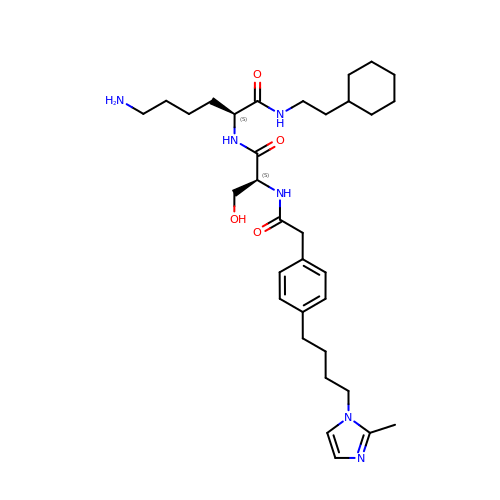[CYCLOHEXYLETHYL]-[[[[4-[2-METHYL-1-IMIDAZOLYL-BUTYL]PHENYL]ACETYL]-SERYL]-LYSINYL]-AMINE | C33 H52 N6 O4 | WHLPIOSHBKQGHA-KYJUHHDHSA-N> DGDQCETSPCQNQG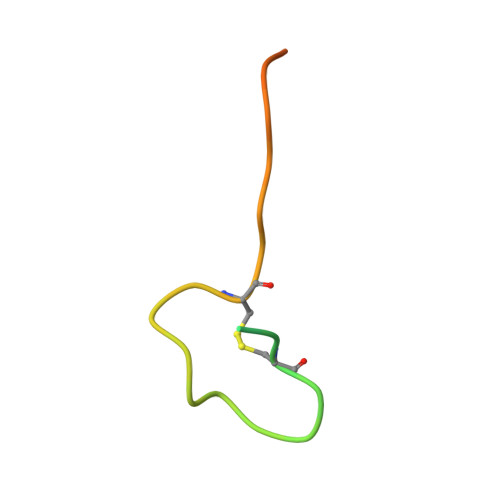KCKDGLGEYTCTCLEGFEGKNCELF> FELLVSFLNTPKYGTFDPTPVVPVFFPFWFGMIVGDIGYALLFYLVGRWLSGYVKRNEPLVIDLFALKLKPQVIGKLVHILNWMVFWTVVWGVIYGEFFGTFLEHLGVFGTPEHPGLIPILIHRIDTAKTANLLILLSVAFGVVLVFFGLALRAYLGLKHRHMAHFWEGVGYLGGLVGVLALAASYLGNLQAGWLQGLMYLGFGVFLLAVLMSRIWLMIPEIFTQAGHILSHIRIYAVGAAGGILAGLLTDV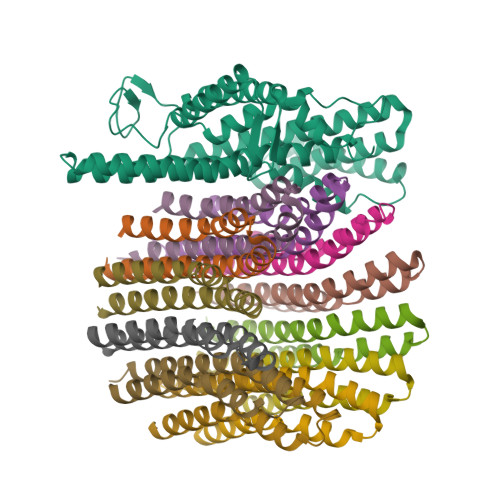GFALAERLGLLGVLLGLLVAGVLHLLILLLTTLGHMLQPIRLLWVEFFTKFGFYEE;>[12x]SGGLDRGLIAVGMGLAVGLAALGTGVAQARIGAAGVGAIAEDRSNFGTALIFLLLPETLVIFGLLIAFILNGRL> SNAMSKTVHYLKDYQTPAYHILKTDLHFDINEPQTVVKSRLTVEPQRVGEPLVLDGSAKLLSVKINGAAADYVLEGETLTIAGVPSERFTVEVETEILPAENKSLMGLYASGGNLFTQCEPEGFRKITFYIDRPDVMSKFTTTIVADKKRYPVLLSNGNKIDGGEFSDGRHWVKWEDPFSKPSYLFALVAGDLAVTEDYFTTMSGRNVKIEFYTTEADKPKVGFAVESLKNAMKWDETRFGLEYDLDIFMVVAVGDFNMGAMENKGLNIFNTKFVLADSRT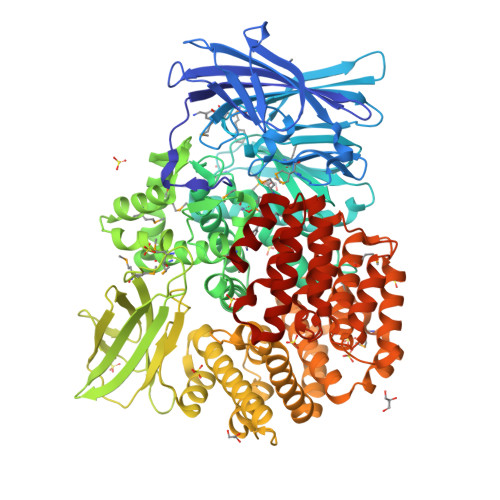ATDTDFEGIESVVGHEYFHNWTGNRVTCRDWFQLSLKEGLTVFRDQEFSGDRASRAVRRIENIRLLRQHQFPEDAGPTAHPVRPASYEEMNNFYTMTVYEKGAEVVRMYHTLLGEEGFQKGMKLYFQRHDGQAVTCDDFRAAMADANGINLDQFALWYSQAGTPVLEAEGRLKNNIFELTVKQTVPPTPDMTDKQPMMIPVKVGLLNRNGEAVAFDYQGKRATEAVLLLTEAEQTFLLEGVTEAVVPSLLRGFSAPVHLNYPYSDDDLLLLLAHDSDAFTRWEAAQTLYRRAVAANLATLSDGVELPKHEKLLAAVEKVISDDLLDNAFKALLLGVPSEAELWDGAENIDPLRYHQAREALLDTLAVHFLPKWHELNRQAAKQENQSYEYSPEAAGWRTLRNVCRAFVLRADPAHIETVAEKYGEMAQNMTHEWGILSAVNGNESDTRNRLLAQFADKFSDDALVMDKYFALVGSSRRSDTLQQVRTALQHPKFSLENPNKARSLIGSFSRNVPHFHAEDGSGYRFIADKVIEIDRFNPQVAARLVQAFNLCNKLEPHRKNLVKQALQRIRAQEGLSKDVGEIVGKILD MnSOD-2 and MnSOD-3 are homologous proteins and are both synthesized as precursors with N-terminal mitochondrial targeting signals. Here we present the structures of the two MnSODs which are strikingly similar to that from human. Gel-filtration chromatography indicated that the pure proteins were tetrameric, a result that was confirmed by analytical ultracentrifugation (results not shown). Similar to other reported MnSODs, the tetrameric quaternary structure in MnSOD-2 and MnSOD-3 is accomplished through interactions of the N-domain α-hairpin.

MnSOD-3 is associated with diapause and its expression is induced in the long-lived dauer stage. Dissection of the insulin/IGF signalling pathway has identified sod-3 as a significant target for the DAF-16/FOXO transcription factor. Inhibition of the insulin/IGF signalling pathway results in elevated expression of sod-3 and an extension in lifespan. A second MCAC purification yielded MnSOD-2 to 70% purity, while further ion exchange of MnSOD-3 using CM-52 gave a sample that was 98% pure. Specific activity was estimated for MnSOD-2 as 3622 ± 80 U mg−1 per manganese and for MnSOD-3 as 3261 ± 26 U mg−1 per manganese; the proteins were 60 and 100% metallated with mangan­ese, respectively. The C. elegans MnSODs are structurally similar to the human enzyme; superposition of all the Cα atoms of MnSOD-2 and MnSOD-3 with human SOD gives root-mean-square-deviations of 0.5 and 0.8 Å, respectively. One chain (chain C) in each SOD asymmetric unit was found to contain electron density corresponding to the N-terminal methionine residue. Two cis-prolines (Pro16) are present in each chain in common with other MnSODs.

>[2x]MKHTLPDLPFDYADLEPVISHEIMQLHHQKHHATYVNNLNQIEEKLHEAVSKGNLKEAIALQPALKFNGGGHINHSIFWTNLAKDGGEPSKELMDTIKRDFGSLDNLQKRLSDITIAVQGSGWGWLGYCKKDKILKIATCANQDPLEGMVPLFGIDVWEHAYYLQYKNVRPDYVHAIWKIANWKNISERFANARQ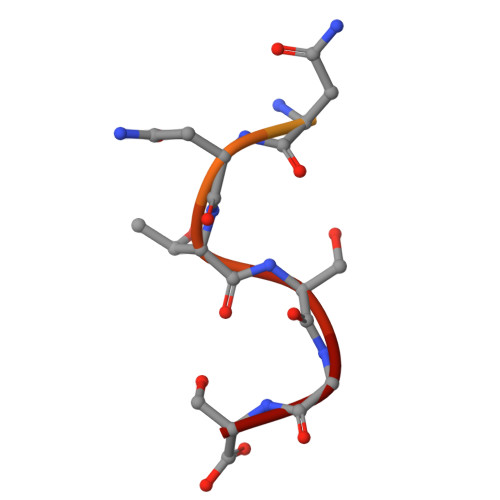> HSVNQRFGSNNTSGS> GSHMKFPGKRKSKHYFPVNARDPLLQQFQPENE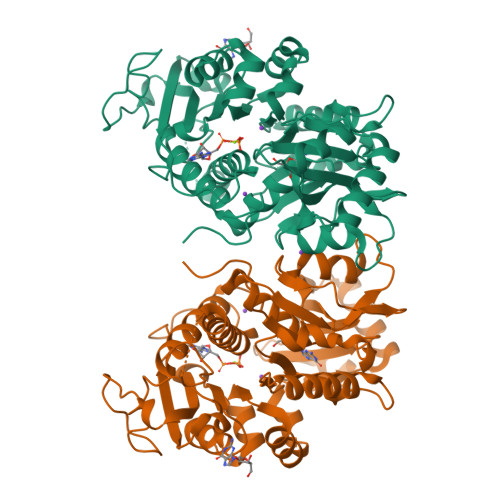TSAAWVVGIDQTLVDIEAKVDDEFIERYGLSAGHSLVIEDDVAEALYQELKQKNLITHQFAGGTIGNTMHNYSVLADDRSVLLGVMCSNIEIGSYAYRYLCNTSSRTDLNYLQGVDGPIGRCFTLIGESGERTFAISPGHMNQLRAESIPEDVIAGASALVLTSYLVRCKPGEPMPEATMKAIEYAKKYNVPVVLTLGTKFVIAENPQWWQQFLKDHVSILAMNEDEAEALTGESDPLLASDKALDWVDLVLCTAGPIGLYMAGFTEDEAKRKTQHPLLPGAIAEFNQYEFSRAMRHKDCQNPLRVYSHIAPYMGGPEKIMNTNGAGDGALAALLHDITANSYHRSNVPNSSKHKFTWLTYSSLAQVCKYANRVSYQVLNQHSPRLTRGLPEREDSLEESYWDR> MAIPEEFDILVLGGGSSGSCIAGRLANLDHSLKVGLIEAGENNLNNPWVYLPGIYPRNMKLDSKTASFYTSNPSPHLNGRRAIVPCANVLGGGSSINFMMYTRGSASDYDDFQAEGWKTK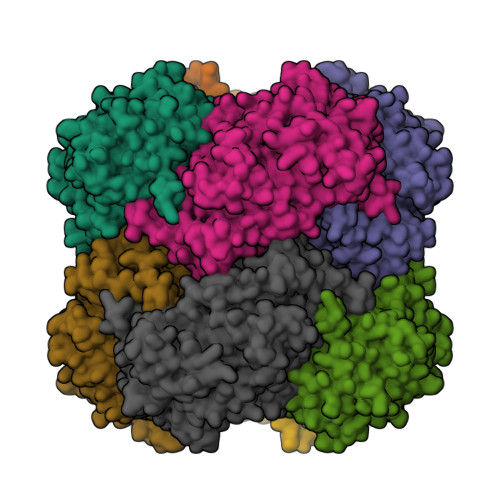DLLPLMKKTETYQRACNNPDIHGFEGPIKVSFGNYTYPVCQDFLRASESQGIPYVDDLEDLVTAHGAEHWLKWINRDTGRRSDSAHAFVHSTMRNHDNLYLICNTKVDKIIVEDGRAAAVRTVPSKPLNPKKPSHKIYRARKQIVLSCGTISSPLVLQRSGFGDPIKLRAAGVKPLVNLPGVGRNFQDHYCFFSPYRIKPQYESFDDFVRGDAEIQKRVFDQWYANGTGPLATNGIEAGVKIRPTPEELSQMDESFQEGYREYFEDKPDKPVMHYSIIAGFFGDHTKIPPGKYMTMFHFLEYPFSRGSIHITSPDPYAAPDFDPGFMNDERDMAPMVWAYKKSRETARRMDHFAGEVTSHHPLFPYSSEARALEMDLETSNAYGGPLNLSAGLAHGSWTQPLKKPTAKNEGHVTSNQVELHPDIEYDEEDDKAIENYIREHTETTWHCLGTCSIGPREGSKIVKWGGVLDHRSNVYGVKGLKVGDLSVCPDNVGCNTYTTALLIGEKTATLVGEDLGYSGEALDMTVPQFKLGTYEKTGLARF> SATRRYYLGAVELSWDYMQSDLGELPVDARFPPRVPKSFPFNTSVVYKKTLFVEFTDHLFNIAKPRPPWMGLLGPTIQAEVYDTVVITLKNMASHPVSLHAVGVSYWKASEGAEYDDQTSQREKEDDKVFPGGSHTYVWQVLKENGPMASDPLCLTYSYLSHVDLVKDLNSGLIGALLVCREGSLAKEKTQTLHKFILLFAVFDEGKSWHSETKNSLMQDRDAASARAWPKMHTVNGYVNRSLPGLIGCHRKSVYWHVIGMGTTPEVHSIFLEGHTFLVRNHRQASLEISPITFLTAQTLLMDLGQFLLFCHISSHQHDGMEAYVKVDSCPEEPQLRMKNNEEAEDYDDDLTDSEMDVVRFDDDNSPSFIQIRSVAKKHPKTWVHYIAAEEEDWDYAPLVLAPDDRSYKSQYLNNGPQRIGRKYKKVRFMAYTDETFKTREAIQHESGILGPLLYGEVGDTLLIIFKNQASRPYNIYPHGITDVRPLYSRRLPKGVKHLKDFPILPGEIFKYKWTVTVEDGPTKSDPRCLTRYYSSFVNMERDLASGLIGPLLICYKESVDQRGNQIMSDKRNVILFSVFDENRSWYLTENIQRFLPNPAGVQLEDPEFQASNIMHSINGYVFDSLQLSVCLHEVAYWYILSIGAQTDFLSVFFSGYTFKHKMVYEDTLTLFPFSGETVFMSMENPGLWILGCHNSDFRNRGMTALLKVSSCDKNTGDYYEDSYEDISAYLLSKNNAIEPRS;> DPLAWDNHYGTQIPKEEWKSQEKSPEKTAFKKKDTILSLNACESNHAIAAINEGQNKPEIEVTWAKQGRTERLCSQNPPVLKRHQREITRTTLQSDQEEIDYDDTISVEMKKEDFDIYDEDENQSPRSFQKKTRHYFIAAVERLWDYGMSSSPHVLRNRAQSGSVPQFKKVVFQEFTDGSFTQPLYRGELNEHLGLLGPYIRAEVEDNIMVTFRNQASRPYSFYSSLISYEEDQRQGAEPRKNFVKPNETKTYFWKVQHHMAPTKDEFDCKAWAYSSDVDLEKDVHSGLIGPLLVCHTNTLNPAHGRQVTVQEFALFFTIFDETKSWYFTENMERNCRAPCNIQMEDPTFKENYRFHAINGYIMDTLPGLVMAQDQRIRWYLLSMGSNENIHSIHFSGHVFTVRKKEEYKMALYNLYPGVFETVEMLPSKAGIWRVECLIGEHLHAGMSTLFLVYSNKCQTPLGMASGHIRDFQITASGQYGQWAPKLARLHYSGSINAWSTKEPFSWIKVDLLAPMIIHGIKTQGARQKFSSLYISQFIIMYSLDGKKWQTY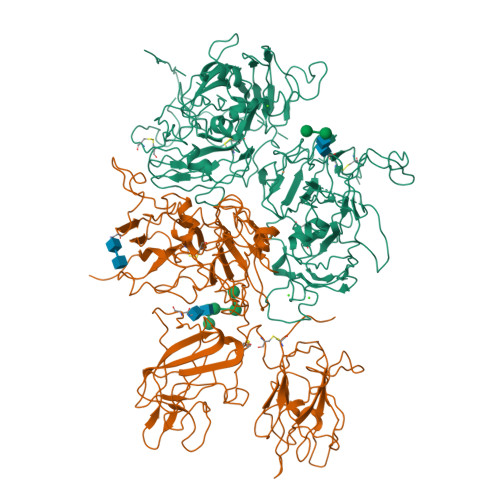RGNSTGTLMVFFGNVDSSGIKHNIFNPPIIARYIRLHPTHYSIRSTLRMELMGCDLNSCSMPLGMESKAISDAQITASSYFTNMFATWSPSKARLHLQGRSNAWRPQVNNPKEWLQVDFQKTMKVTGVTTQGVKSLLTSMYVKEFLISSSQDGHQWTLFFQNGKVKVFQGNQDSFTPVVNSLDPPLLTRYLRIHPQSWVHQIALRMEVLGCEAQDLY In plants, DNA methylation occurs in CG, CHG, and CHH contexts (where H = A, T, or C), with the maintenance of CG methylation mediated by the DNA methyltransferase MET1. MET1 possesses replication foci target sequence (RFTS) 1–2, acidic-linker, bromo adjacent homology (BAH) 1–2 and methyltransferase (MTase) domains, whereas DNMT1 possesses PCNA-binding, RFTS, CXXC, autoinhibitory linker, BAH1-2 and MTase domains. Of note, MET1 has two RFTS domains and lacks the CXXC domain. Arabidopsis thaliana MET1 exhibits a plant-specific structural feature in the autoinhibition state, and a conserved activation state compared to mammalian DNMT1.

To uncover the activation state of MET1, we determined the cryo-EM structure of MET1MTase bound to 12 bp hemimethylated DNA in which the target cytosine in hemimethylation site was replaced by a 5-fluorocytosine (5fC) to form an irreversible covalent complex with MET1. Cryo-EM map of the MET1MTase bound to hemimethylated DNA complex was successfully reconstructed at 2.74 Å resolution, which enables us to generate the atomic model of the complex, except for the acidic-linker (aa: 646–707), loops and linkers in BAH1 (aa: 748–751), and BAH2 (aa: 925–933, 958–965, 1050–1054 and 1059–1089). Domain assembly of the BAH1, BAH2 and MTase domains of MET1 was similar to that of DNMT1, with root mean square deviation (RMSD) of 0.768 Å over 682 aligned Cα atoms, indicating the conserved rigid core structure. The MTase domain of MET1 consists of two moieties, catalytic core containing S-adenosyl homocysteine (SAH, a methyl donor cofactor product) binding site and target recognition domain (TRD: 1305–1477). Hemimethylated DNA was sandwiched by the catalytic core and TRD, in which TRD loop1 (aa:1426-1434) interacted with the backbone phosphates of the non-target strand of the DNA. In addition, the main chain carbonyl of Met1461 and side chain of Lys1463 in TRD loop2 (aa: 1458–1470) interacted with 5-methylcytosine (5mC) and the adjacent guanin in 5mCG of the non-target strand, respectively. The methyl group of 5mC in the non-target strand was tightly surrounded by Cys1427, Leu1428, Trp1438, Leu1441, Met1461 and Gly1462 of the TRD via van der Waals interactions. Flipped-out 5fC in the target strand was covalently bound to sulfhydryl group of Cys1198 of the catalytic loop in MET1 (aa: 1196–1210), and recognized by side chains of Glu1238, Arg1282 and Arg1284 of the catalytic core, in which side chain of Met1204 occupies the vacant space after base flipping of 5fC. The spatial positions of the 5fC and 5mC bases in the hemimethylated DNA were strictly restricted by the catalytic loop and TRD, respectively, which ensure the robust CG sequence methylation of MET160. In the N-terminal region of MET1, the Activating Helix (aa: 631–644) was adpted to a helix-turn conformation, which is similar to the conformation of the Activating Helix in the activation state of DNMT149.

> GPLGSKRKAMQATTTRLVNRIWGEFYSNYSPEDPLQATAAENGEDEVEEEGGNGEEEVEEEGENGLTEDTVPEPVEVQKPHTPKKIRGSSGKREIKWDGESLGKTSAGEPLYQQALVGGEMVAVGGAVTLEVDDPDEMPAIYFVEYMFESTDHCKMLHGRFLQRGSMTVLGNAANERELFLTNECMTTQLKDIKGVASFEIRSRPWGHQYRKKNITADKLDWARALERKVKDLPTEYYCKSLYSPERGGFFSLPLSDIGRSSGFCTSCKIREDEEKRSTIKLNVSKTGFFINGIEYSVEDFVYVNPDSIGGLKEGSKTSFKSGRNIGLRAYVVCQLLEIVPKESRKADLGSFDVKVRRFYRPEDVSAEKAYASDIQELYFSQDTVVLPPGALEGKCEVRKKSDMPLSREYPISDHIFFCDLFFDTSKGSLKQLPANMKPKFSTIKDDTLLRKKKGKGVESEIESEIVKPVEPPKEIRLATLDIFAGCGGLSHGLKKAGVSDAKWAIEYEEPAGQAFKQNHPESTVFVDNCNVILRAIMEKGGDQDDCVSTTEANELAAKLTEEQKSTLPLPGQVDFINGGPPCQGFSGMNRFNQSSWSKVQCEMILAFLSFADYFRPRYFLLENVRTFVSFNKGQTFQLTLASLLEMGYQVRFGILEAGAYGVSQSRKRAFIWAAAPEEVLPEWPEPMHVFGVPKLKISLSQGLHYAAVRSTALGAPFRPITVRDTIGDLPSVENGDSRTNKEYKEVAVSWFQKEIRGNTIALTDHICKAMNELNLIRCKLIPTRPGADWHDLPKRKVTLSDGRVEEMIPFCLPNTAERHNGWKGLYGRLDWQGNFPTSVTDPQPMGKVGMCFHPEQHRILTVRECARSQGFPDSYEFAGNINHKHRQIGNAVPPPLAFALGRKLKEALHLKKSPQHQP>[3x]PMFI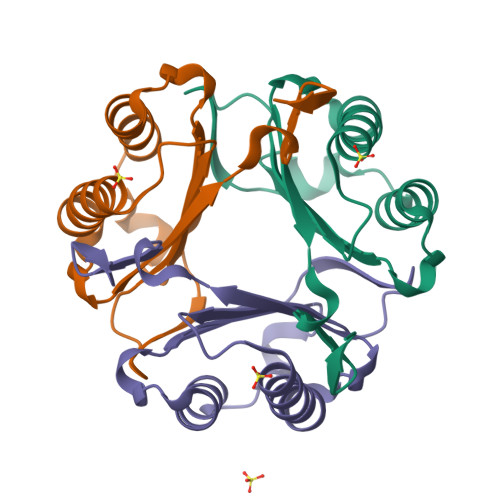VNTNVPRASVPDGFLSELTQQLAQATGKPPQYIAVHVVPDQFMAFGGSSEPCALCSLHSIGKIGGAQNRSYSKLLCGLLAERLRISPDRVYINYYDMNAANVGWNNSTFA>[4x]MKETRDLETLSVNAIRFLAIDAVEKARSGHPGMPMGMAPLAYLLFREVMRHNPLDPDWPDRDRFVLSAGHGSMLLYAVLHLTGYDLPLEELKSFRQWGSKTPGHPERGHTPGVEVTTGPLGQGISTAVGLALAERKLAAEFNRPGHVVVDHYTYVLASDGDLMEGVSGEAASLAGHWGLSKLIVFWDDNRISIDGPTDLAFTEDVLARYRAYGWQTLRVEDVNDLEALRKAIKLAKLDERPTLIAVRSHIGFGSPKQDSAKAHGEPLGPEAVEATRRN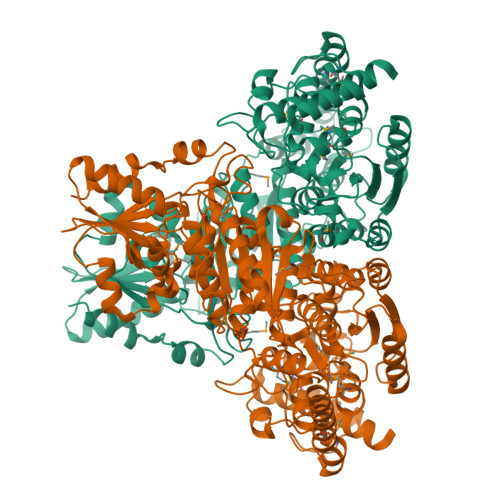LGWPYPPFVVPEEVYRHMDMREKGRAWQEAWEKALEAYARAYPDLHQELMRRLRGELPPLPEEPPSFDKPIATRAASGRALNLLAPRLPELLGGSADLTPSNNTKAEGMEDFSRANPLGRYLHFGVREHAMGAILNGLNLHGGYRAYGGTFLVFSDYMRPAIRLAALMGVPTVFVFTHDSIALGEDGPTHQPVEHLMSLRAMPNLFVIRPADAYETFYAWLVALRRKEGPTALVLTRQAVPLLSPEKARGLLRGGYVLEDVEEPQGVLVATGSEVHLALRAQALLREKGVRVRVVSLPSFELFAAQPEAYRKEVLPPGLPVVAVEAGASLGWERYAHKVVALDRFGASAPYPEVYERLGFTPERVAEAFLSLV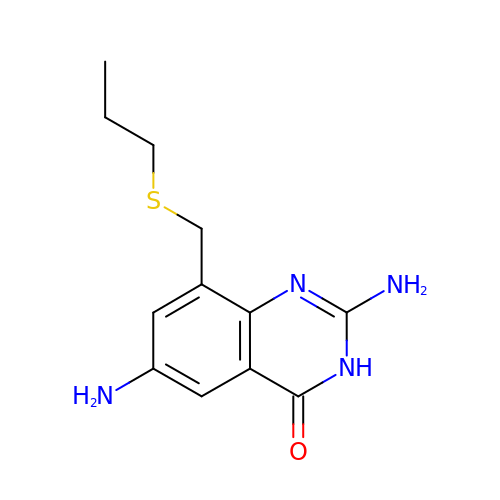2,6-DIAMINO-8-PROPYLSULFANYLMETHYL-3H-QUINAZOLINE-4-ONE | C12 H16 N4 O S | RSKNEWMEOVQZII-UHFFFAOYSA-N(11alpha,14beta)-11,17,21-trihydroxypregn-4-ene-3,20-dione 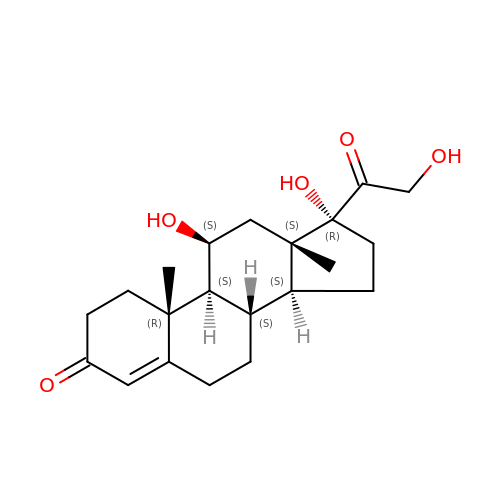| C21 H30 O5 | JYGXADMDTFJGBT-VWUMJDOOSA-N> MGIDINTKIFNSVAEVFQKAQGSYAGHRKHIAVLKKIQSKAVEQGYEDAFNFWFDKLVTKILPLKKNEIIDRIVKLVAAFIASLERELILAKKQNYKLTNDEEGIFSRFVDQFIRHVLRGVESPDKNVRFRVLQLLAVIMDNIGEIDESLFNLLILSLNKRIYDREPTVRIQAVFCLTKFQDEEQTEHLTELSDNEENFEATRTLVASIQNDPSAEVRRAAMLNLINDNNTRPYILERARDVNIVNRRLVYSRILKSMGRKCFDDIEPHIFDQLIEWGLEDRELSVRNACKRLIAHDWLNALDGDLIELLEKLDVSRSSVCVKAIEALFQSRPDILSKIKFPSIWKDFTVEIAFLFRAIYLYCLDNNITEMLEENFPEASKLSEHLNHYILLRYHHNDISNDSQSHFDYNTLEFIIEQLSIAAERYDYSDEVGRRSMLTVVRNMLALTTLSEPLIKIGIRVMKSLSINEKDFVTMAIEIINDIRDDDIEKQESESDIINNLPPEKEASSATIVLCLTRSSYMLELVNTPLTENILIASLMDTLITPAVRNTAPNIRELGVKNLGLCCLLDVKLAIDNMYILGMCVSKGNASLKYIALQVIVDIFSVHGNTVVDGEGKVDSISLHKIFYKVLKNNGLPECQVIAAEGLCKLFLADV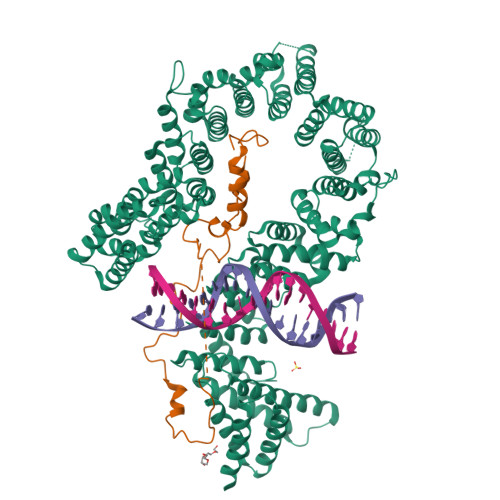FTDDDLFETLVLSYFSPINSSNEALVQAFAFCIPVYCFSHPAHQQRMSRTAADILLRLCVLWDDLQSSVIPEVDREAMLKPNIIFQQLLFWTDPRNLVNQTGSTKKDTVQLTFLIDVLKIYAQIEKKEIKKMIITNINAIFLSSEQDYSTLKELLEYSDDIAENDNLDNVSKNALDKLRNNLNSLIEEINERSETQTKDENNTANDQYSSILGN;> GPLGHMSIFEKDLMAYFDENLNRNWRGREHWKVRNFKKANLVNKESDLLEETRTTIGDTTDKNTTDDKSMDTKKKHKQKKVLEIDFFKTDDSFEDKVFASKGRTKIDMPIKNRKNDTHYLLPDDFHFSTDRITRLFIKPGQKMSLFSHRKHT> MFRAAAPGQLRRAASLLRFQSTLVIAEHANDSLAPITLNTITAATRLGGEVSCLVAGTKCDKVAQDLCKVAGIAKVLVAQHDVYKGLLPEELTPLILATQKQFNYTHICAGASAFGKNLLPRVAAKLEVAPISDIIAIKSPDTFVRTIYAGNALCTVKCDEKVKVFSVRGTSFDAAATSGGSASSEKASSTSPVEISEWLDQKLTKSDRPELTGAKVVVSGGRGLKSGENFKLLYDLADQLHAAVGASRAAVDAGFVPNDMQVGQTGKIVAPELYIAVGISGAIQHLAGMKDSKTIVAINKDPEAPIFQVADYGIVADLFKVVPEMTEILKKK;> MAELRVLVAVKRVIDYAVKIRVKPDRTGVVTDGVKHSMNPFCEIAVEEAVRLKEKKLVKEVIAVSCGPAQCQETIRTALAMGADRGIHVEVPPAEAERLGPLQVARVLAKLAEKEKVDLVLLGKQAIDDDCNQTGQMTAGFLDWPQGTFASQVTLEGD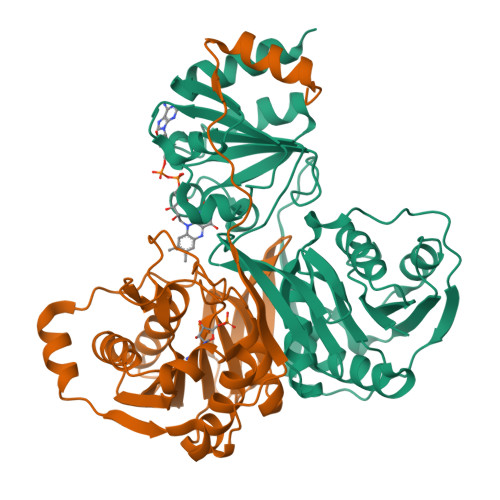KLKVERAIDGGLETLRLKLPAVVTADLRLNEPRYATLPNIMKAKKKKIEVIKPGDLGVDLTSKLSVISVEDPPQRTAGVKVETTEDLVAKLKEIGRI>[2x]SAPAQEHPEATVLFSDIVGFTEIASRSSPLEVCSLL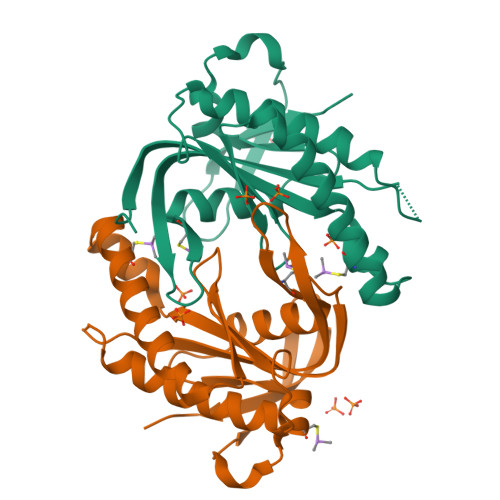DELYQRFDAAIEEYPQLYKVETIGDAYMVVCNVTVPCDDHADVLLEFALRMHEEASRVASSLGEPVRIRVGMHSGPVVAGVVGRKMPRFCLFGDTVNTASRMESHGEAGQIHISEACYCCLRSKERFEIRERGNITVKGKGTMRTYLLSPLERT> GMADEATRRVVSEIPVLKTNAGPRDRELWVQRLKEEYQSLIRYVENNK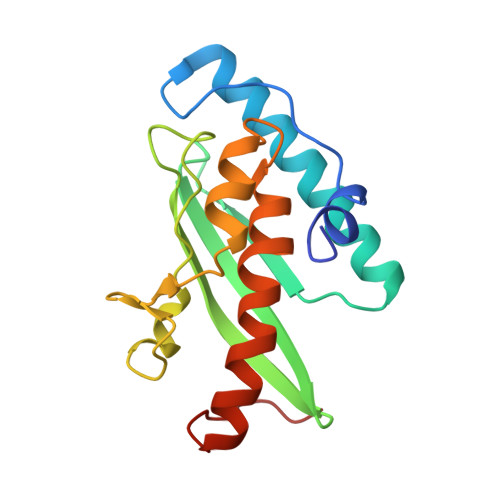NADNDWFRLESNKEGTRWFGKCWYIHDLLKYEFDIEFDIPITYPTTAPEIAVPELDGKTAKMYRGGKICLTDHFKPLWARNVPKFGLAHLMALGLGPWLAVEIPDLIQKGVIQHKEKCNQ> MKIYVDGREVIINDNERNLLEALKNVGIEIPNLCYLSEASIYGACRMCLVEINGQITTSCTLKPYEGMKVKTNTPEIYEMRRNILELILATHNRDCTTCDRNGSCKLQKYAEDFGIRKIRFEALKKEHVRDESAPVVRDTSKCILCGDCVRVCEEIQGVGVIEFAKRGFESVVTTAFDTPLIETECVLCGQCVAYCPTGALSIRNDIDKLIEALESDKIVIGMIAPAVRAAIQEEFGIDEDVAMAEKLVSFLKTIGFDKVFDVSFGADLVAYEEAHEFYERLKKGERLPQFTSCCPAWVKHAEHTYPQYLQNLSSVKSPQQALGTVIKKIYARKLGVPEEKIFLVSFMPCTAKKFEAEREEHEGIVDIVLTTRELAQLIKMSRIDINRVEPQPFDRPYGVSSQAGLGFGKAGGVFSCVLSVLNEEIGIEKVDVKSPEDGIRVAEVTLKDGTSFKGAVIYGLGKVKKFLEERKDVEIIEVMACNYGCVGGGGQPYPNDSRIREHRAKVLRDTMGIKSLLTPVENLFLMKLYEEDLKDEHTRHEILHTTYRPRRRYPEKDVEILPVPNGEKRTVKVCLGTSCYTKGSYEILKKLVDYVKENDMEGKIEVLGTFCVENCGASPNVIVDDKIIGGATFEKVLEELSKNG;> MFKNAKEFVQYANKLKTLREKKLNGVSIYVCVGTGCTAKGALKVYSAFEEELKKRNLLGQVTLEKIDDDKVTLNRTGCCGRCSSGPLVKIMPYRFFYSNVAPEDVPEIVDRTVLKGEPIERLFLTDPLTGEKVPRIEDTTLFKNQDFYIMEAIGESECDSIEDYIARSGYESLVKALTSMTPEEIIETVKASGLRGRGGGGFPTGLKWEFTRKAQGDIKFVVCNGDEGDPGA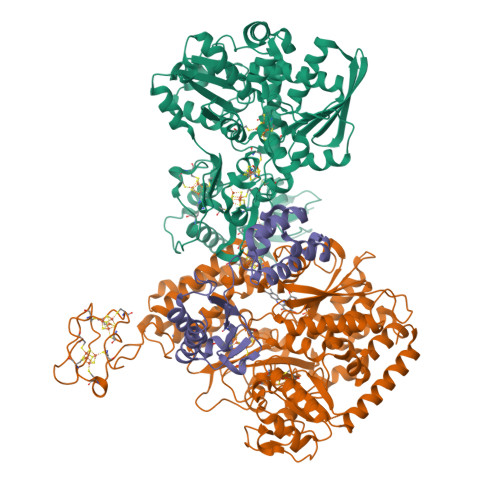FMNRTLLERDPHLVLEGMIIAGYAVGAQKGYAYIRAEYPFAVKMFKKAIEDARKLGLLGENILGTGFSFDLEVKEGAGAFVCGEETALLASIEGKRGMPRPKPPFPAQSGLWGKPTLINNVETYANIPRILRDGVENYRKRGTENSPGTKMFSVAGPLKATGIIEVEFGTTLRDIIYNICGGFVEGEEFKAVQIGGPSGACLSEDFIDMPLDYDTLKKADAMVGSGGIVVITKKTCMVEVARFFLDFTKRESCGKCVPCREGTMQAYNILEKFTHGKATYEDLKTLEHLSKTIKTASLCGLGKTAPNPILSTLKLFREEYIAHIEGECPSGMCTAFKKYVINPDICKGCGLCARSCPQNAITGERGKPYTIDQEKCVKCGLCASKCPFKAIELV;> MASWSHPQFEKSGGGGGENLYFQGAVLALERHFEKVEEILKKYGYKRENLIKILLEIQEIYRYLPEDVINYVSTAMGIPPAKIYGVATFYAQFSLKPKGKYTIMVCDGTACHMAGSPEVLKAIEEETGLTPGNVTEDLMFSLDQVGCLGACALAPVMVINGEVYGNLTADKVKEILRKIKEKERESANV>GAMGSPKEHIDLYQQIKWNGWGDTRKFLHQLKPSGTIAMTTPEVSSVPLPSLRGFIKKELTLPGEEDKPFVLDETPALQIENIHVDPPKQYPEFVRELKAFFLPDQLKDDKLARITHTFGKSLRDLIRVRIGQVKNAPDLIVLPHSHEEVERLVQLAHKYNVVIIPMGGGSNIVGAIEPVSNERFTVSIDMRRMNKVLWVDRREMTACIQVGIMGPELEKQLHKQGVSLGHDPDSFEFSTLGGWLATCSSGHQSDKYGDIEDMAVSFRTVTPTGTLELRNGARSGAGINYKHIILGSEGTLGIITEAVMKVHAVPQAVEYYGFLFPTFAHAVSALQQIRSSEVIPTMIRVYDPEETQLSFAWKPSKGAVSEFTSAMVKKYLHYIRSFDFKNVCLSIIGFEGPKKVVDFHRTSVFDILSKNAAFGLGSAPGKTWAEKRYDLPYIRDFLLDHNMWVDVAETTVSYANLQTLWKDAKQTFVKHFKDQGIPAWICAHISHTYTNGVCLYFIFASKQNENKDMAQYIEAKKLMTDIIFKYGGSLSHHHGVGYEHVPWMTRYATRGWINVYRSLKET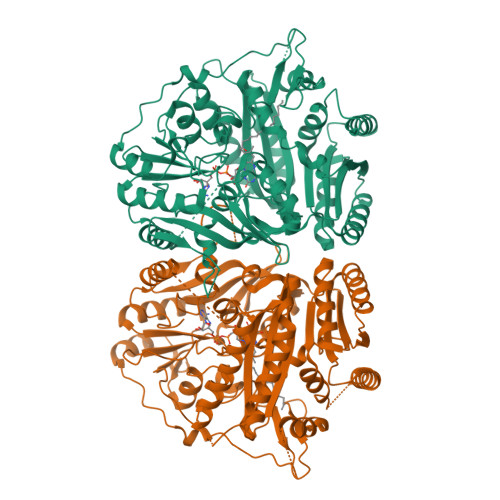IDPKDICNPRKLI[4x]>GGTDINKLIEEGKKHYLPKTYTFDNGKIIIKAGDKVEESKIQKLYWASKEVKSQFHRIIGNDKPLEVGNADDILTIVIYNNPEEYKLNKTLYGYSVDNGGIYIEGIGTFFTYERTPQESIYSLEELFRHEFTHYLQGRYLIPGLFNKGDFYKGNNGRITWFEEGSAEFFAGSTRTSVLPRKSMVGGLSKNPKERFNADKLLHSKYSDGWDFYKYGYAFSDYMYNNNKKLFSDLVSTMKNNDVKGYEALIEESSKDSKINKDYEYHMENLVNNYDNYTIPLVSDDYMKQYDNKSLHEIKSDIEKAMDVKNSQITKESSQYFDTYNLKATYTLSSNKGEISNWNYMNNKINEALNKLDNLSWGGYKTVTAYFSN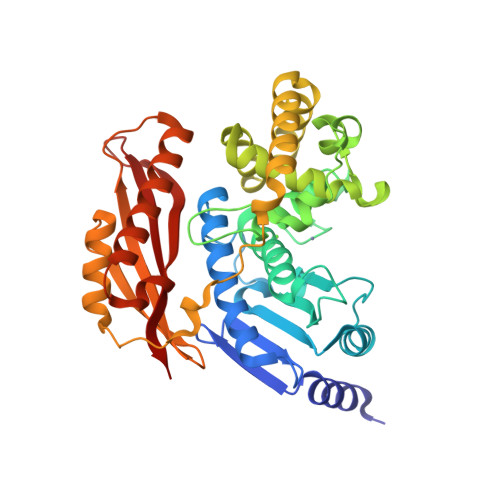PRLNSNNEVVYDIVFHGLLSHN[2x]1-[(4-chlorophenyl)methyl]-4-(3-imidazol-1-ylpropyl)piperazin-2-one 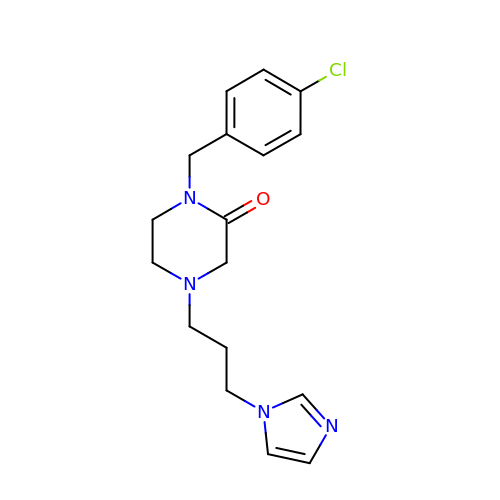| C17 H21 Cl N4 O | UHJVZFXZSLURRR-UHFFFAOYSA-N>SMKIFNKESLNQLEKKGYLIIDNFLNDLNKINLIYDESYNQFKENKLIEAGMNKGTDKWKDKSIRGDYIQWIHRDSNSRIQDKDLSSTIRNINYLLDKLDLIKNEFDNVIPNFNSIKTQTQLAVYLNGGRYIKHRDSFYSSESLTISRRITMIYYVNKDWKKGDGGELRLYTNNPNNTNQKELKQTEEFIDIEPIADRLLIFLSPFLEHEVLQCNFEPRIAITTWIY[3x]

PHD homologues exist in other types of eukaryotes and prokaryotes where they act on non HIF substrates. The respective prolyl-hydroxylases (DdPhyA and TgPhyA) catalyze prolyl-hydroxylation of S-phase kinase-associated protein 1 (Skp1), a reaction enabling adaptation to different dioxygen availability. In the cellular slime mold Dictyostelium discoideum, the human parasite Toxoplasma gondii and the crop pathogen Pythium ultimum, PHD-type 2OG oxygenases catalyze the hydroxylation of a prolyl residue in the S-phase kinase-associated protein (Skp1). This enables Skp1 glycosylation in a manner proposed to regulate protein degradation via effects on the SCF class of E3-ubiquitin ligase of which Skp1 is an essential subunit; however, glycosylation independent roles of Skp1 prolyl hydroxylation are also manifested.

Following construct optimization and use of thermal shift assays, which revealed that Ni(II) ions and N-oxalylglycine (a stable 2OG analog) stabilize the enzymes, we obtained crystals of DdPhyA(60-284) (space group C2221, 3 molecules per asymmetric unit, resolution 2.02 Å) from which we were able to determine a structure by molecular replacement. Consistent with all reported 2OG oxygenase structures, DdPhyA contains an eight stranded “distorted” DSBH (βI-βVIII) core-fold. The structure has three disordered regions (Asn134–Leu142 (finger loop), Asn230–Glu244 (β5(IV)/β6(V) loop), and Arg161–Arg174 ((II)–β4(III) loop)). Each of these disordered loops is likely involved in substrate binding, as is the case for some other 2OG oxygenases (see below). The DdPhyA active site contains three protein metal ion ligands, i.e. His191, Asp193, and His266, which form the conserved HXD…H motif present in most, but not all, 2OG oxygenases. Octahedral coordination of the nickel ion (substituting for iron) is completed by a water molecule and the oxalyl group of NOG, the latter in a bidentate manner. The C-5 carboxylate of NOG is bound via a salt bridge involving both its oxygens with the Arg276 guanidino group and via one of its oxygens with the Tyr212 alcohol. Although there are minor differences, e.g. in the precise 2OG methylene/NOG NH positions, the geometry of the metal ion and NOG/2OG-binding elements of DdPhyA are strikingly similar to those observed in HsPHD2 and TaPHD. Notably, the C terminus of DdPhyA is much shorter than all other prolyl hydroxylases for which structures are available, i.e. it is truncated at the end of β9 (VIII, C-terminal residue: Tyr284). The results for DdPhyA, however, demonstrate that an extended prolyl hydroxylase C terminus is not necessary for efficient coupling of 2OG turnover with substrate oxidation.> TIFQFPQDFMWGTATAAYQIEGAYQEDGRGLSIWDTFAHTPGKVFNGDNGNVACDSYHRYEEDIRLMKELGIRTYRFSVSWPRIFPNGDGEVNQKGLDYYHRVVDLLNDNGIEPFCTLYHWDLPQALQDAGGWGNRRTIQAFVQFAETMFREFHGKIQHWLTFNEPWCIAFLSNMLGVHAPGLTNLQTAIDVGHHLLVAHGLSVRRFRELGTSGQIGIAPNVSWAVPYSTSEEDKAACARTISLHSDWFLQPIYQGSYPQFLVDWFAEQGATVPIQDGDMDIIGEPIDM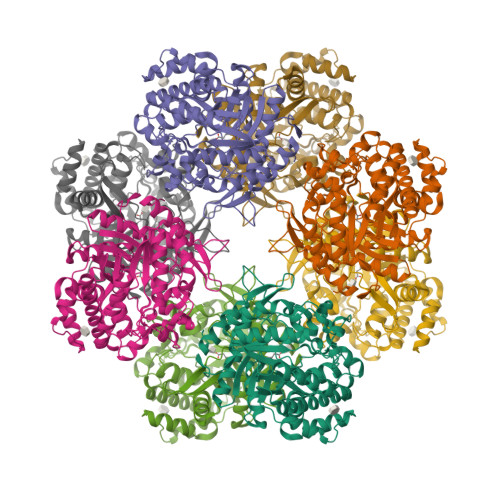IGINYYSMSVNRFNPEAGFLQSEEINMGLPVTDIGWPVESRGLYEVLHYLQKYGNIDIYITENGACINDEVVNGKVQDDRRISYMQQHLVQVHRTIHDGLHVKGYMAWSLLDNFEWAEGYNMRFGMIHVDFRTQVRTPKQSYYWYRNVVSNNWLETRR>[2x]GPAMKNARRVSLSPLILRSLAELQDGLNTVVDKNWRQLRRPGDWSLAITMEAAELLDSYPWKWWKNVKAQPDLQNVKIELTDILHFSLSGAMQVSDENSGAVHKAEAGSNGESGKHWCYFDQPRALPA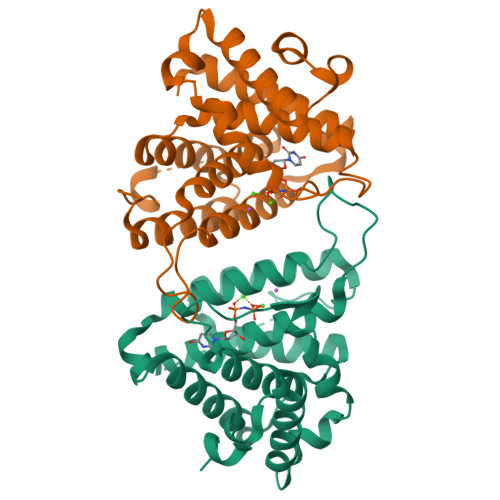AGGAEYVACVETPGSSLSAPVSADECDLADFMFFPLSDTNNALASFQNIIRLASLQRFQLVTSAVIAAADDIGFNLVAYYVAKHTLNGIRQMKGYKDGTYVKVQKGVEDNELLHGCISPFSLDDVTNEGNYKTKWDDIMHRVYDAFGTPKEERLNIGHWLKS> EK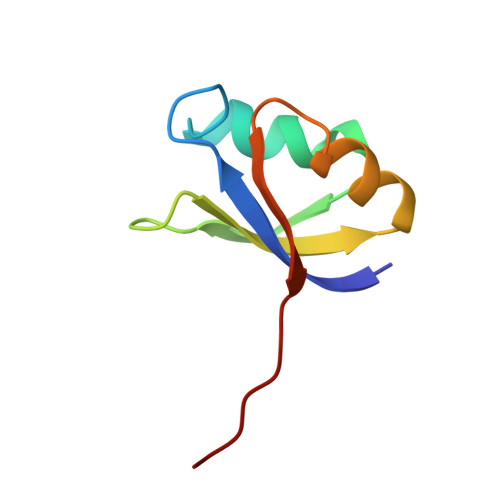KYIVGFKQTMSAMSSAKKKDVISQKGGKVEKQFKYVNAAAATLDEKAVKELKKDPSVAYVEEDHIAHEY>SMSTLLINQPQYAWLKELGLREENEGVYNGSWGGRGEVITTYCPANNEPIARVRQASVADYEETVKKAREAWKIWADIPAPKRGEIVRQIGDALREKIQVLGSLVSLEMGKILVEGVGEVQEYVDICDYAVGLSRMIGGPILPSERSGHALIEQWNPVGLVGIITAFNFPVAVYGWNNAIAMICGNVCLWKGAPTTSLISVAVTKIIAKVLEDNKLPGAICSLTCGGADIGTAMAKDERVNLLSFTGSTQVGKQVGLMVQERFGRSLLELGGNNAIIAFEDADLSLVVPSALFAAVGTAGQRCTTARRLFIHESIHDEVVNRLKKAYAQIRVGNPWDPNVLYGPLHTKQAVSMFLGAVEEAKKEGGTVVYGGKVMDRPGNYVEPTIVTGLGHDASIAHTETFAPILYVFKFQNEEEVFAWNNEV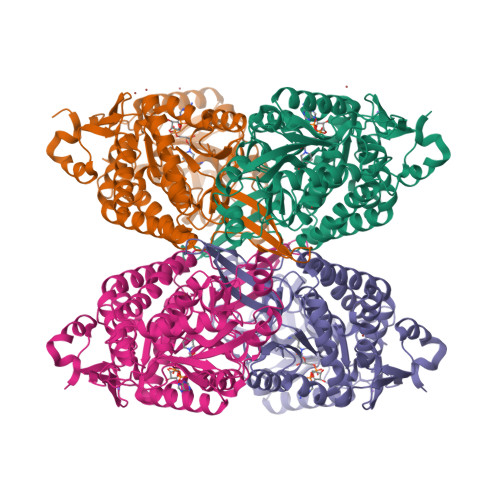KQGLSSSIFTKDLGRIFRWLGPKGSDCGIVNVNIPTSGAEIGGAFGGEKHTGGGRESGSDAWKQYMRRSTCTINYS[8x]> GSHMKNSVSVDLPGSMKVLVSKSSNADGKYDLIATVDALELSGTSDKNNGSGVLEGVKADASKVKLTISDDLGQTTLEVFKSDGSTLVSKKVTSKDKSSTYELFNEKGELSLKYITRADKSSTYELFNEKGELSLKYITRADKSSTYELFNEKGELSEKKITRADKSSTYELFNEKGELSLKYITRADGTRLEYTGIKSDGSGKAKEVLKGYVLEGTLTAEKTTLVVKEGTVTLSKNISKSGEVSVELNDTDSSAATKKTAAWNSGTSTLTITVNSKKTKDLVFTSSNTITVQQYD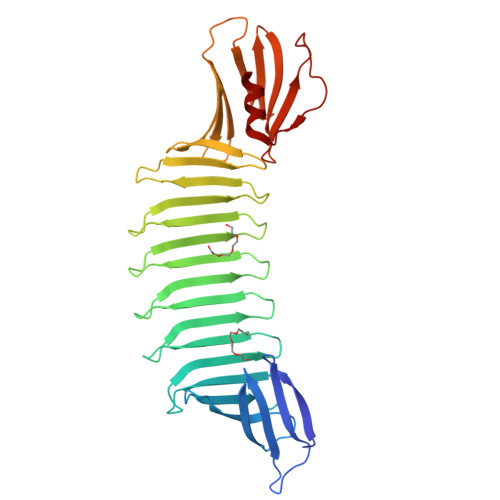SNGTSLEGSAVEITKLDEIKNALK> GSHMASMSKDEVKREAKDTDGNPEIKGERRRLH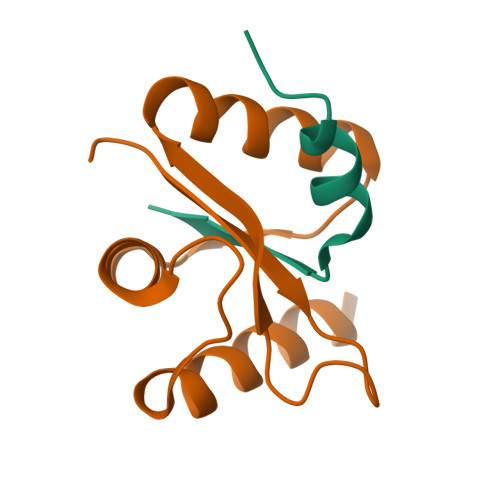SEIQSGSLANNIKKSTVIVKN;> PTHIAICLYYKLGETPLPLVIETGKDAKALQIIKLAELYDIPVIEDIPLATSLYKNIHKGQYITEDFFEPVAQLIRIAIDLDY(~{E})-3-(1,3-benzothiazol-2-yl)-4-(4-methoxyphenyl)but-3-enoic 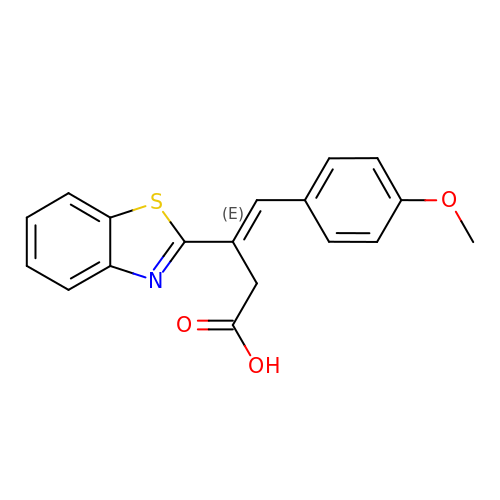acid | C18 H15 N O3 S | SONSOTYJHQIJQV-JLHYYAGUSA-N>[2x]MGSSHHHHHHSQDPMLSVGATTTATRLTGWGRTAPSVANVLRTPDAEMIVKAVARVAESGGGRGAIARGLGRSYGDNAQNGGGLVIDMTPLNTIHSIDADTKLVDIDAGVNLDQLMKAALPFGLWVPVLPGTRQVTVGGAIACDIHGKNHHSAGSFGNHVRSMDLLTADGEIRHLTPTGEDAELFWATVGGNGLTGIIMRATIEMTPTSTAYFIADGDVTASLDETIALHSDGSEARYTYSSAWFDAISAPPKLGRAAVSRGRLATVEQLPAKLRSEPLKFDAPQLLTLPDVFPNGLANKYTFGPIGELWYRKSGTYRGKVQNLTQFYHPLDMFGEWNRAYGPAGFLQYQFVIPTEAVDEFKKIIGVIQASGHYSFLNVFKLFGPRNQAPLSFPIPGWNICVDFPIKDGLGKFVSELDRRVLEFGGRLYTAKDSRTTAETFHAMYPRVDEWISVRRKVDPLRVFASDMARRLELL

DprE1 is the first of two enzymes that catalyze the conversion of decaprenylphosphoryl-β-D-ribose (DPR) to decaprenylphosphoryl-β-D-arabinose (DPA). In its natural context, DprE1 catalyzes the oxidation of the 2′ hydroxyl group of DPR to give the ketone decaprenylphosphoryl-2-keto-β-D-erythropentofuranose (DPX), with flavin adenine dinucleotide (FAD) acting as the oxidant in the reaction. After BTZs have entered the catalytic pocket of DprE1 containing the reduced form of the flavin cofactor (FADH2), which was generated by oxidation of the substrate, the nitro group of the BTZs is reduced to nitroso which can then form a covalent bond with a nearby cysteine residue (Cys387, Mtb enzyme numbering). We obtained co-crystal structures of Mtb-DprE1 with BTZ compounds 1, 2, 9, and 12 and BOZ compound 5.

Compounds 1 and 8 are the two-electron reduced forms of 7 and 12, respectively, also referred to as nitroso. We were interested to compare the kinetics of inactivation of DprE1 by 1 and 8, which do not require activation, relative to the BTZ counterparts, 7 and 12, that require reductive activation. Unbiased difference density maps, calculated with phases from structure models prior to incorporation of the ligand, demonstrated that all five compounds formed a covalent bond with the active site cysteine (Cys387). The nitroso-BTZ 1 bound in the same way that CT325 did, corroborating the ability of CT325 to serve as a BTZ substitute. For instance, the planes of the BTZ scaffold of compounds 1 and 5 enclose an angle of 15°, with the other three compounds in between these two extremes. The complexes with BTZ and BOZ inhibitors induce partial ordering of the 315–330 loop in some cases (compounds 1, 2 and 12). We used the nitroso-BTZ (1) and hydroxylamino-BTZ (2) as positive controls, which demonstrated that a +343 Da species is detected by mass spectrometry and therefore any trace of this species, if it occurred with 11, would have been observed.In this paper, we report the crystal structures of a lectin from Agrocybe aegerita, designated as AAL2, in its apo- and complex forms with GlcNAc and GlcNAcβ1-3Galβ1-4GlcNAc, as part of our endeavors to develop a system to facilitate the identification and purification of O-GlcNAcylated proteins. AAL2 was recently discovered from the fruit body of the edible mushroom A. aegerita. AAL2 was found to specifically bind nonreducing terminal N-acetylglucosamine (GlcNAc) moieties of either alpha- or beta-linkage and was reported to have the activity of inducing apoptosis in hepatoma cells in vitro as well as inhibiting hepatoma growth in tumour-bearing mice in vivo. The overall structure of AAL2 monomer is a single domain with the shape of cylindrical torus with a diameter of about 51Å and a height of about 27Å, showing a very regular, seven-bladed β-propeller fold formed by the blades packing in a circular array.

The structures of AAL2, AAL2-GlcNAc and AAL2-GlcNAcβ1-3Galβ1-4GlcNAc were determined at resolutions of 2.0Å, 2.1Å, and 2.0Å, respectively. There are two virtually identical AAL2 monomers arranged around a two-fold pseudoaxis of symmetry in an asymmetric unit in both the structures of AAL2 and AAL2-GlcNAc, and one AAL2 monomer in AAL2-GlcNAcβ1-3Galβ1-4GlcNAc, while the protein exists as monomers in solution as determined from its elution volume on a Superdex 200 10/300 GL column. The ligands we used were GlcNAc monosaccharide and GlcNAcβ1-3Galβ1-4GlcNAc, a trisaccharide showing very high affinity toward AAL2 in glycan array analysis. GlcNAcβ1-3Galβ1-4GlcNAc ligands are bound to the same pockets of AAL2, with the non-reducing terminal GlcNAc (1’-GlcNAc) adopted the same position as GlcNAc. The interactions between AAL2 and 1’-GlcNAc of the trisaccharide are identical to those with GlcNAc monosaccharide. Although there are several hydrogen bond interactions between AAL2, such as Lys138, and the LacNAc moiety after 1’-GlcNAc, AAL2 doesn’t demonstrate specific preference to the 2’-Gal or 3’-GlcNAc in all the six blades, since the interactions seem to be random. This result was rather unexpected based on the glycan array. However, our results have further proved that AAL2 recognizes the terminal non-reducing GlcNAc moiety of a polysaccharide. AAL2 was also shown via SPR to bind to the trisaccharide with a Kd value of 41.65 μM, which is close to that of GlcNAc, demonstrating that Gal-GlcNAc moiety beyond GlcNAc may not affect the binding between AAL2 and trisaccharide.

> TSNVITQDLPIPVASRGFADIVGFGLDGVVIGRNAVNLQPFLAVKNFAQNAGGWLTTKHVRLIADTTGTGKGDIVGFGNAGVYVSVNNGKNTFADPPKMVIANFGYDAGGWRVEKHLRYLADIRKTGRADIIGFGEKGVLVSRNNGGLNFGPATLVLKDFGYDAGGWRLDRHLRFLADVTGNGHLDIVGFGDKHVFISRNNGDGTFAPAKSVIDNFCIDAGGWKIGDHPRFVADLTGDGTADIIGCGKAGCWVALNNGGGVFGQVKLVINDFGTDKGWQAAKHPRFIADLTGNGRGDVVGFGNAGVYVALNNGDGTFQSAKLVLKDFGVQQGWTVSKHRRFVVDLTGDGCADIIGFGEKETLVSYNDGKGNFGPVKALTNDFSFSGGKWAPETTVCWMANLDSSRH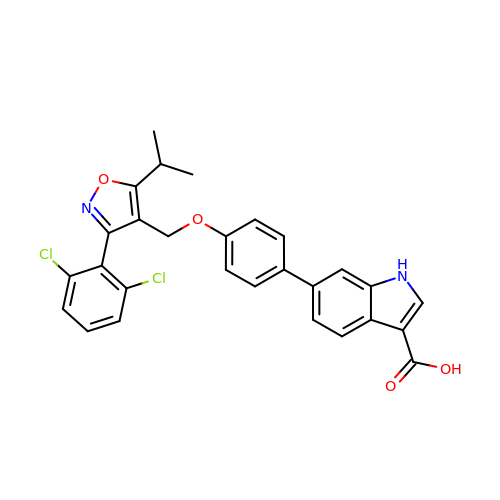6-(4-{[3-(2,6-dichlorophenyl)-5-(propan-2-yl)-1,2-oxazol-4-yl]methoxy}phenyl)-1H-indole-3-carboxylic acid | C28 H22 Cl2 N2 O4 | MUZVVRUJHSGOMN-UHFFFAOYSA-N Here we studied metal-preference evolution within the natural diversity of the iron/manganese superoxide dismutase (SodFM) family of reactive oxygen species scavengers. Only a few metalloenzymes have been rigorously demonstrated to be cambialistic in vivo, including some iron (Fe)- or manganese (Mn)-dependent superoxide dismutases (SODs; SodFMs); metalloenzymes that play an important role in cellular reactive oxygen species defence. To study this process, we leveraged the existence of naturally Fe-specific, Mn-specific and flexible Fe/Mn-cambialistic SodFM homologues, which differentially utilize these metals to catalyse the detoxification of superoxide. By combining phylogenetics, biochemistry and structural biology, we demonstrate that SodFM metal utilization can be evolutionarily fine tuned by sliding along a scale between perfect manganese and iron specificities.

a,b, Residues at the XD-2 position in cambialistic S. aureus SodFM1 (LD-2, a) and B. fragilis SodFM2 (GD-2, b) were mutated to those found commonly at this position in natural SodFMs. In the cambialistic SodFM2 from B. fragilis (b), all mutants displayed lower activity with Mn and the majority had higher activity with Fe, representing change towards its most likely ancestral Fe-preferring phenotype. c, For Fe-preferring CPR Wolfebacteria SodFM1 (CPR-His), mutations in both the XD-2 and water-coordinating H/Q residues were necessary to shift towards the inferred ancestral higher Mn activity. The likely ancestral phenotype was proxied by the closely related SodFM1 from more basal Wolfebacteria. g,h, Single mutants, but not double mutants, shifted metal preference of N. alba SodFM3 (g, Q/H mutant) and Woesearchaeota SodFM4 (h, VD-2A). d–f, Crystal structures of S. aureus SodFM1 LD-2G (d), B. fragilis SodFM2 GD-2T (e) and CPR-His SodFM1 VD-2G H/Q double mutant (f) were analyzed to investigate structural effects of these mutations. The structures in e and f were solved in this study. Importantly, consistent with previous reports, comparison of four protein crystal structures of the WT and mutant SodFMs we determined here indicated that metal-preference modulation by XD-2 and Q/H occurs without any significant changes to the secondary metal coordination sphere within the resolution limits of the solved structures. This provides further support for ‘redox tuning’ via subtle structural changes.

>[6x]MYEMPKLPYANNALEPVISQQTIDYHYGKHLQTYVNNLNSLVPGTEYEGKTVEAIVASAPDGAIFNNAGQVLNHTLYFLQFAPKPAKNEPAGKLGEAIKRDFGSFENFKKEFNAASVGLFGSGWAWLSVDKDGKLHITKEPNGSNPVRAGLKPLLTCDVWEHAYYLDYQNRRADHVNKLWEIIDWDVVEKRL> MAQINASYQRDMAIALPGMVADTSKYNIDGACVVNEGDVLVGAAVQVVQAQAVDGHKLVKALTTGTTPYGVAIRSHWQTVNAQNQMIYEDGGA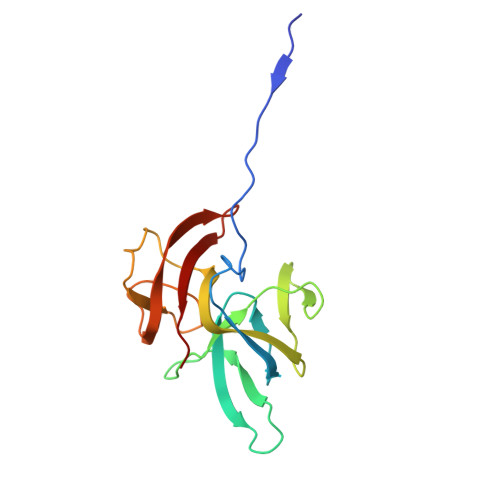INVMTSGRVWMLSKSTEAPTFGSAVKLDVDGQEKSDGTIETTWTYAGGWTKYKDIQLVEVQLHQL>[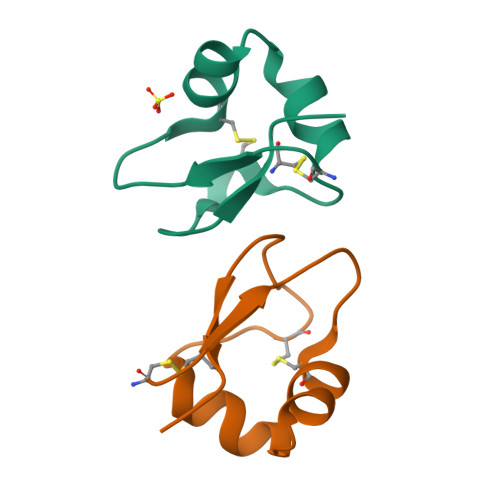2x]ACTSYYTVKSGDICYNIAQTYGIDVATLQSYNPGLQCDNLQIGQQLCVAD>ASKTAVVDVKGAVANPGVYEVAADARVRDAIALAGGLTDEADETKVNLAAKVHDEMMIYVPKKGEDAPASNAVSKSPSDGDRNGMQVAINTATEEELMQLPGIGPAKA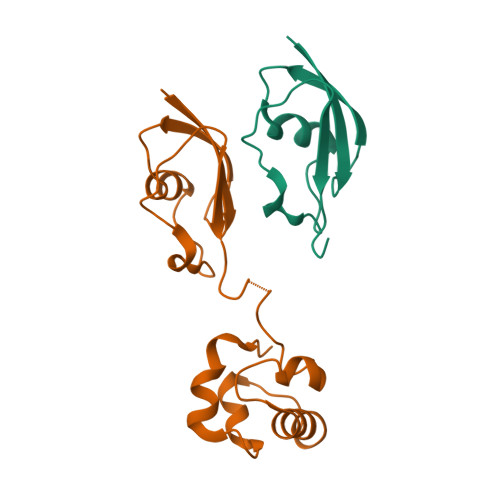NAIIAYREEHGPFRRVEDLLNVTGIGEKTLEKLKPYLLVP[2x]> GAMGRILFLTTFMSKGNKVVRYLESLHHEVVICQEKVHAQSANLQEIDWIVSYAYGYILDKEIVSRFRGRIINLHPSLLPWNKGRDPVFWSVWDETPKGVTIHLIDEHVDTGDILVQEEIAFADEDTLLDCYNKANQAIEELFIREWENIVHGRIAPYRQTAGGTLHFKADRDFYKNLNMTTVRELLALKRLCAEPKRGEKPIDKTFHQLFEQQVEMTPDHVAVVDRGQSLTYKQLNERANQLAHHLRGKGVKPDDQVAIMLDKSLDMIVSILAVMKAGGAYVPIDPDYPGERIAYMLADSSAAILLTNALHEEKANGACDIIDVHDPDSYSENTNNLPHVNRPDDLVYVMYTSGSTGLAKGVMIEHHNLVNFCEWYRPYFGVTPADKALVYSSFSFDGSALDIFTHLLAGAALHIVPSERKYDL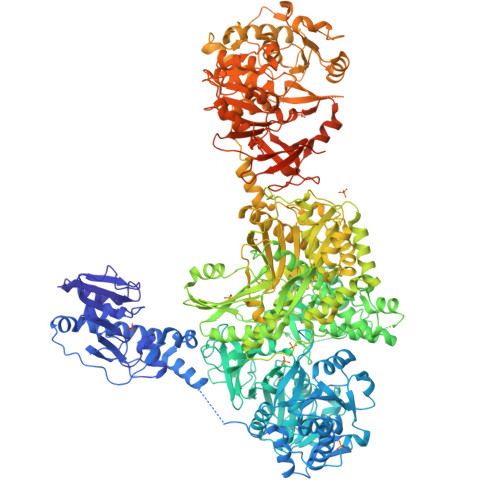DALNDYCNQEGITISYLPTGAAEQFMQMDNQSFRVVITGGDVLKKIERNGTYKLYNGYGPTECTIMVTMFEVDKPYANIPIGKPIDRTRILILDEALALQPIGVAGELFIVGEGLGRGYLNRPELTAEKFIVHPQTGERMYRTGDRARFLPDGNIEFLGRLDNLVKIRGYRIEPGEIEPFLMNHPLIELTTVLAKEQADGRKYLVGYYVAPEEIPHGELREWLGNDLPDYMIPTYFVHMKAFPLTANGKVDRRALPDVQADAELLGEDYVAPTDELEQQLAQVWSHVLGIPQMGIDDHFLERGGDSIKVMQLIHQLKNIGLSLRYDQLFTHPTIRQLKRLLTEQKQVSLEPLRELDEQAEYETSAVEKRMYIIQQQDVESIAYNVVYTINFPLTVDTEQIRVALEQLVLRHEGLRSTYHMRGDEIVKRIVPRAELSFVRQTGEEESVQSLLAEQIKPFDLAKAPLLRAGVIETADKKVLWFDSHHILLDGLSKSILARELQALLGQQVLSPVEKTYKSFARWQNEWFASDEYEQQIAYWKTLLQGELPAVQLPTKKRPPQLTFDGAIQMYRVNPEITRKLKATAAKHDLTLYMLMLTIVSIWLSKMNSDSNQVILGTVTDGRQHPDTRELLGMFVNTLPLLLSIDHEESFLHNLQQVKAKLLPALQNQYVPFDKILEAARVKREGNRHPLFDVMFMMQGAPETELESNMHHINAGISKFDLTLEVLERENGLNIVFEYNTHLFDEGMILRMVAQFEHLLLQAVHGLDQQVKRFELVTEDEKRDLFLRVNDTAKAYPNKLIMSMLEDWAAATPDKTALVFREQRVTYRELNERVNQLAHTLREKGVQPDDLVMLMAERSVEMMVAIFAVLKAGGAYLPIDPHSPAERIAYIFADSGAKLVLAQSPFVEKASMAEVVLDLNSASSYAADTSNPPLVNQPGDLVYVMYTSGSTGKPKGVMIEHGALLNVLHGMQDEYPLLQDDAFLLKTTYIFDISVAEIFGWVPGRGKLVILEPEAEKNPKAIWQAVVGAGITHINFVPSMLIPFVEYLEGRTEANRLRYILACGEAMPDELVPKVYEVLPEVKLENIYGPTEATIYASRYSLAKGSQESPVPIGKPLPNYRMYIINRHGQLQPIGVPGELCIAGASLARGYLNNPALTEEKFTPHPLEKGERIYRTGDLARYREDGNIEYLGRMDHQVKIRGYRIELDEIRSKLIQEETIQDAVVVARNDQNGQAYLCAYLLSEQEWTVGQLRELLRRELPEYMIPAHFVLLKQFPLTANGKLDRKALPEPDGSVAAAENLYFQ> MEEKEILWNEAKAFIAACYQELGKAAEVKDRLADIKSEIDLTGSYVHTKEELEHGAKMAWRNSNRCIGRLFWNSLNVIDRRDVRTKEEVRDALFHHIETATNNGKIRPTITIFPPEEKGEKQVEIWNHQLIRYAGYESDG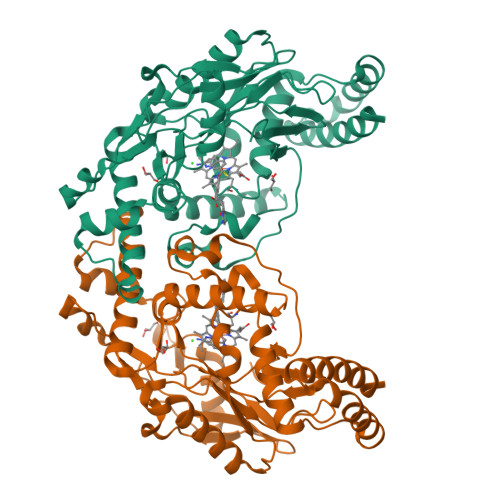ERIGDPASCSLTAACEELGWRGERTDFDLLPLIFRMKGDEQPVWYELPRSLVIEVPITHPDIEAFSDLELKWYGVPIISDMKLEVGGIHYNAAPFNGWYMGTEIGARNLADEKRYDKLKKVASVIGIAADYNTDLWKDQALVELNKAVLHSYKKQGVSIVDHHTAASQFKRFEEQAEEAGRKLTGDWTWLIPPISPAATHIFHRSYDNSIVKPNYFYQDKPYE> KPGAPWWKSAVFYQVYPRSFKDTNGDGIGDFKGLTEKLDYLKGLGIDAIWINPHYASPNTDN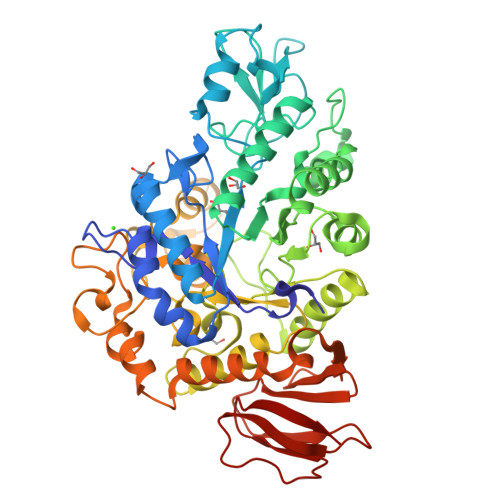GYDISDYREVMKEYGTMEDFDRLMAELKKRGMRLMVDVVINHSSDQHEWFKSSRASKDNPYRDYYFWRDGKDGHEPNNYPSFFGGSAWEKDPVTGQYYLHYFGRQQPDLNWDTPKLREELYAMLRFWLDKGVSGMRFDTVATYSKTPGFPDLTPEQMKNFAEAYTQGPNLHRYLQEMHEKVFDHYDAVTAGEIFGAPLNQVPLFIDSRRKELDMAFTFDLICYDRALDRWHTIPRTLADFRQTIDKVDAIAGEYGWNTFFLGNHDNPRAVSHFGDDRPQWREASAKALATVTLTQRGTPFIFQGDELGMTNYPFKTLQDFDDIEVKGFFQDYVETGKATAEELLTNVALTSRDNARTPFQWDDSANAGFTTGKPWLKVNPNYTEINAAREIGDPKSVYSFYRNLISIRHETPALSTGSYRDIDPSNADVYAYTRSQDGETYLVVVNFKAEPRSFTLPDGMHIAETLIESSSPAAPAAGAASLELQPWQSGIYKVK>MSSSHHHHHHMPTKKQKSKSKLKPFFALVRRTNPSYGKLAFALALSVVTTLVSLLIPLLTKQLVDGFSMSNLSGTQIGLIALVFFVQAGLSAYATYALNYNGQKIISGLRELLWKKLIKLPVSYFDTNASGETVSRVTNDTMVVKELITTHISGFITGIISVIGSLTILFIMNWKLTLLVLVVVPLAALILVPIGRKMFSISRETQDETARFTGLLNQILPEIRLVKASNAEDVEYGRGKMGISSLFKLGVREAKVQSLVGPLISLVLMAALVAVIGYGGMQVSSGELTAGALVAFILYLFQIIMPMGQITTFFTQLQKSIGATERMIEILAEEEEDTVTGKQIENAHLPIQLDRVSFGYKPDQLILKEVSAVIEAGKVTAIVGPSGGGKTTLFKLLERFYSPTAGTIRLGDEPVDTYSLESWREHIGYVSQESPLMSGTIRENICYGLERDVTDAEIEKAAEMAYALNFIKELPNQFDTEVGERGIMLSGGQRQRIAIARALLRNPSILMLDAATSSLDSQSEKSVQQALEVLMEGRTTIVIAHRLSTVVDADQLLFVEK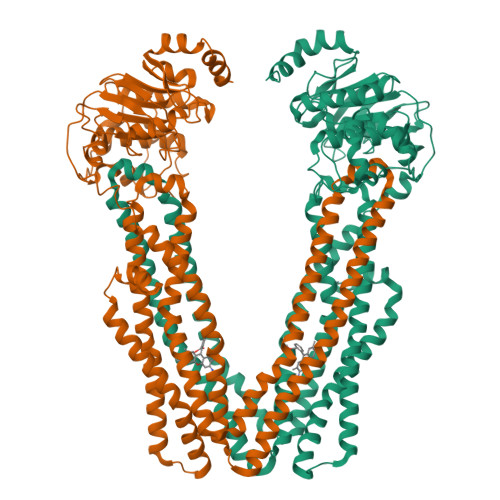GEITGRGTHHELMASHGLYRDFAEQQLKMNADLENKAG[2x]7-chloroquinolin-4-amine | C9 H7 Cl N2 | 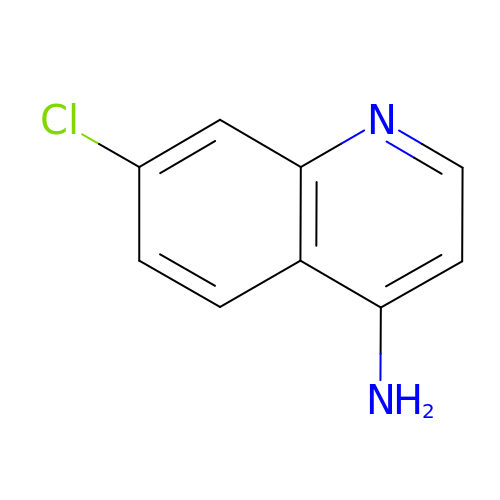NDRZSRWMMUGOBP-UHFFFAOYSA-N4-methyl-3-[(2-pyridin-3-ylpyrido[2,3-d]pyrimidin-4-yl)amino]-~{N}-[3-(trifluoromethyl)phenyl]benzamide | C27 H19 F3 N6 O | 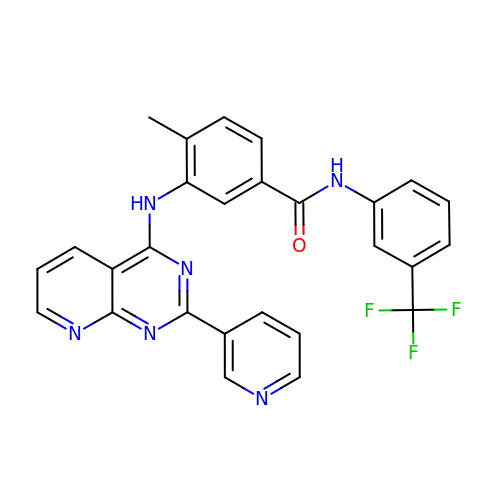SNMQSFPKJXPDDI-UHFFFAOYSA-N>[4x]AEAGITGTWYNQLGSTFIVTAGADGALTGTYEAAVGNAESRYVLTGRYDSAPATDGSGTALGWTVAWKNNYRNAHSATTWSGQYVGGAEARINTQWLLTSGTTEANAWKS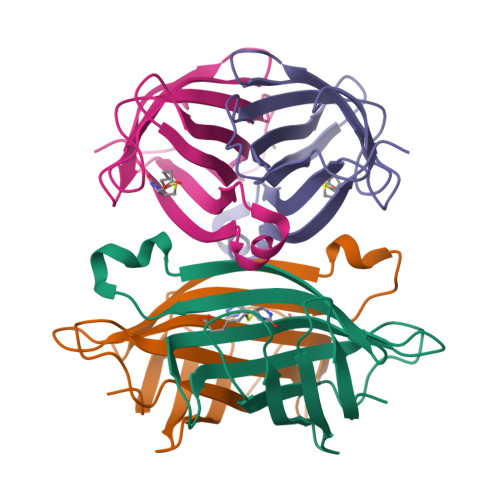TLVGHATFTKVKPSAAS> GSRKGCALLVKLFNGCPLRIHSTAAWTHPSTKDQHLLLGAEEGIFILNRNDQEATLEMLFPSRTTWVYSINNVLMSLSGKTPHLYSHSILGLLERKETRAGNPIAHISPHRLLAAKNMVSTKIQDTKGCRACCVAEGASSGGPFLCGALETSVVLLQWYQPMNKFLLVRQVLFPLPTPLSVFALLTGPGSELPAVCIGVSPGRP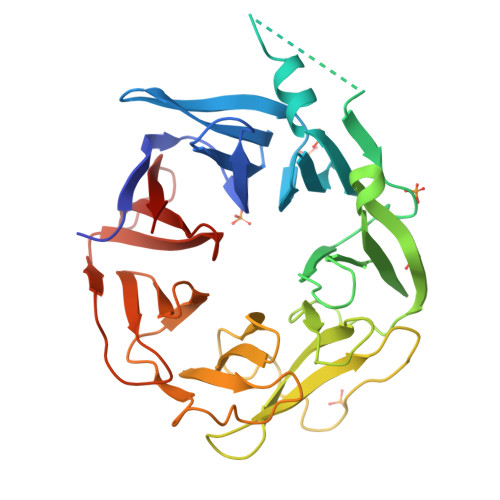GKSVLFHTVRFGALSCWLGEMSTEHRGPVQVTQVEEDMVMVLMDGSVKLVTPEGSPVRGLRTPEIPMTEAVEAVAMVGGQLQAFWKHGVQVWALGSDQLLQELRDPTLTFRLLGSPRPVVVETRPVDDPTAPSNLYIQE Cytosolic purine 5´-nucleotidase (cN-II; EC 3.1.3.5) dephosphorylates purine nucleotide monophosphates with canonical activity towards inosine monophosphate (IMP). The cN-II protein assembles into functional homotetramers, with each subunit comprising 561 amino acid residues. The cN-II structure possesses the overall fold characteristic of the haloacid dehalogenase superfamily: an α/β Rossmann-like “core domain” and a smaller “cap domain. Whole-exome sequencing studies have recently revealed that somatic missense mutations in the gene encoding cN-II (NT5C2) are associated with relapsed acute lymphoblastic leukemia (ALL).

In this study, we describe the biochemical and structural behavior of the three most common mutants: R367Q, R238W, and L375F. Crystals of all three cN-II mutants belonged to the I222 space group with one molecule per asymmetric unit. Overall, the spatial arrangements of the mutants were almost identical to that of the wild type. The L375F mutation is located in alpha-helix 13 (amino acid residues 375–381), which interacts with a 3/10 helix (amino acid residues 485–487) in the neighboring subunit. Introduction of F375 induced a closer contact between the mutated residue and H486 of the adjacent subunit, which was accompanied by a slight displacement of the proximal L379 side chain. Consequently, this led to rearrangement of other surrounding interactions at the oligomeric interface; i.e., the NE1 atom of W382 formed a hydrogen bond with the carbonyl group of H486 in the mutant and with the D487 carbonyl in the wild type. Our data show that the L375F mutation causes local changes at intersubunit contacts. On the other hand, the R238W and L375F mutations stimulated catalytic activity in synergy with ATP binding and caused a decrease in protein thermostability. Interestingly, interface A also includes helix A (amino acid residues 355–365), which was well defined in all the mutant crystal structures. Helix A is formed only in the active state of the cN-II enzyme, and the stabilization of this region in the mutants is consistent with their high catalytic potency even in the absence of ATP.

> MGSSHHHHHHSSGLVPRGSMSTSWSDRLQNAADMPANMDKHALKKYRREAYHRVFVNRSLAMEKIKCFGFDMDYTLAVYKSPEYESLGFELTVERLVSIGYPQELLSFAYDSTFPTRGLVFDTLYGNLLKVDAYGNLLVCAHGFNFIRGPETREQYPNKFIQRDDTERFYILNTLFNLPETYLLACLVDFFTNCPRYTSCETGFKDGDLFMSYRSMFQDVRDAVDWVHYKGSLKEKTVENLEKYVVKDGKLPLLLSRMKEVGKVFLATNSDYKYTDKIMTYLFDFPHGPKPGSSHRPWQSYFDLILVDARKPLFFGEGTVLRQVDTKTGKLKIGTYTGPLQHGIVYSGGSSDTICDLLGAKGKDILYIGDHIFGDILKSKKRQGWRTFLVIPEFAQELHVWTDKSSLFEELQSLDIFLAELYKHLDSSSNERPDISSIQRRIKKVTHDMDMCYGMMGSLFRSGSRQTLFASQVMRYADLYAASFINLLYYPFSYLFRAAHVLMPHESTVEHTHVDINEMESPLATRNRTSVDFKDTDYKRHQLTRSISEIKPPNL> MKKQNPWIYLNEEEKNQIL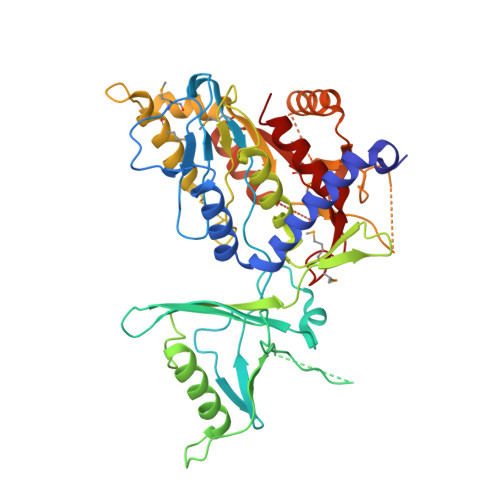NFSESYKKFISKFKTEREVTAYALDKAKKLGFINAEEKKNLMPGDKIFYTCREKSVAFAIIGKNPIEDGMNFIVSHTDSPRLDAKPSPISEENELTFIKTNYYGGIKKYQWLSTPLSIRGVVFLKNGEKVEINIGDNENDPVFVIPDILPHLDRKIQRNKKSDEIVEGENLKILIGSLPIETKEKNKVKLATLQLIKEKYKIEEEDFVSSEIEIVPAGTAKDVGFDKALIGAYGQDDKICVFTSLESIFDLEETPNKTAICFLVDKEEIGSTGSTGLDSRYLEYFVSDMIFKIKKSEYNNLHVQKALWNSKSISADVCAAINPLFSSVHDEQNAPQLGYGIPIMKYTGHGGKSMASDADAELVSYIRQLLNKNNIAWQVATLGKVEEGGGGTVAKFLAGYGIRTIDMGPAVISMHSPMEITSKFDLYNAYLAYKAFYRE5'-O-(N-(L-CYSTEINYL)-SULFAMOYL)ADENOSINE 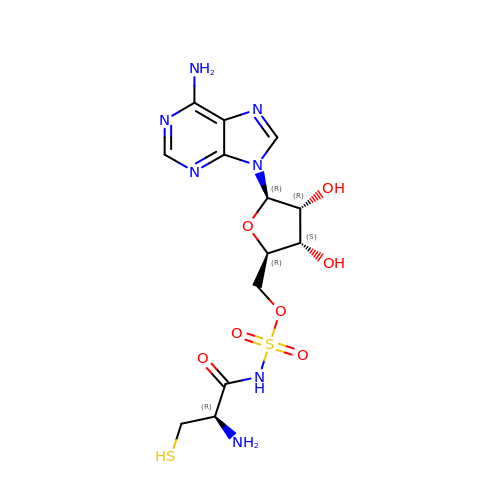| C13 H19 N7 O7 S2 | FTSDEWPMACCNGN-YTMOPEAISA-N>GMHSITENTSWNKEFSAEAVNGVFVLCKSSSKSCATNDLARASKEYLPASTFKIPNAIIGLETGVIKNEHQVFKWDGKPRAMKQWERDLTLRGAIQVSAVPVFQQIAREVGEVRMQKYLKKFSYGNQNISGGIDKFWLEDQLRISAVNQVEFLESL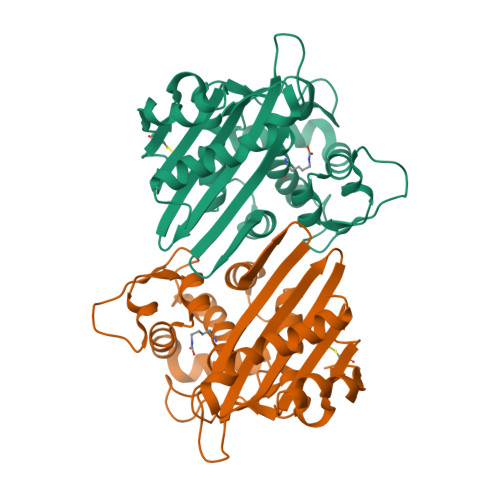YLNKLSASKENQLIVKEALVTEAAPEYLVHSKTGFSGVGTESNPGVAWWVGWVEKETEVYFFAFNMDIDNESKLPLRKSIPTKIMESEGIIG[2x]> MIVSDIEANALLESVTKFHCGVIYDYSTAEYVSYRPSDFGAYLDALEAEVARGGLIVFHNGHKYDVPALTKLAKLQLNREFHLPRENCIDTLVLSRLIHSNLKDTDMGLLRSGKLPGALEAWGYRLGEMKGEYKDDFKRMLEEQGEEYVDGMEWWNFNEEMMDYNVQDVVVTKALLEKLLSDKHYFPPEIDFTDVGYTTFWSESLEAVDIEHRAAWLLAKQERNGFPFDTKAIEELYVELAARRSELLRKLTETFGSWYQPKGGTEMFCHPRTGKPLPKYPRIKTPKVGGIFKKPKNKAQREGREPCELDTREYVAGAPYTPVEHVVFNPSSRDHIQKKLQEAGWVPTKYTDKGAPVVDDEVLEGVRVDDPEKQAAIDLIKEYLMIQKRIGQSAEGDKAWLRYVAEDGKIHGSVNPNGAVTGRATHAFPNLAQIPGVRSPYGEQCRAAFGAEHHLDGITGKPWVQAGIDASGLELRCLAHFMARFDNGEYAHEILNGDIHTKNQIAAELPTRDNAKTFIYGFLYGAGDEAIGQIVGAGKERGKELKKKFLENTPAIAALRESIQQTLVESSQWVAGEQQVKWKRRWIKGLDGRKVHVRSPHAALNTLLQSAGALICKLWIIKTEEMLVEKGLKHGWDGDFAYMAWVHDEIQVGCRTEEIAQVVIETAQEAMRWVGDHWNF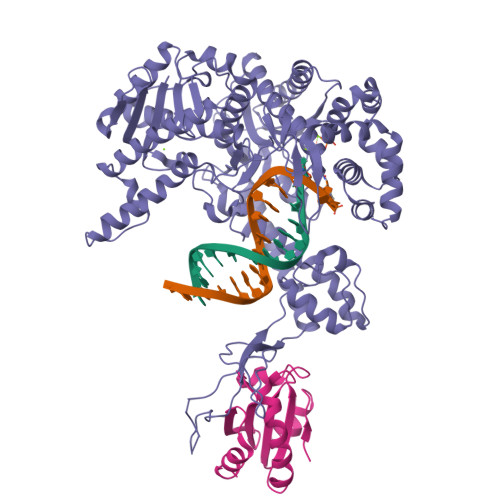RCLLDTEGKMGPNWAICH;> SDKIIHLTDDSFDTDVLKADGAILVDFWAEWCGPCKMIAPILDEIADEYQGKLTVAKLNIDQNPGTAPKYGIRGIPTLLLFKNGEVAATKVGALSKGQLKEFLDANLA>SHMMVSQETVAHVKDLIGQKEVFVAAKTYCPYSKATLSTLFQELNVPKSKALVLELDEMSNGSEIQDALEEISGQKTVPNV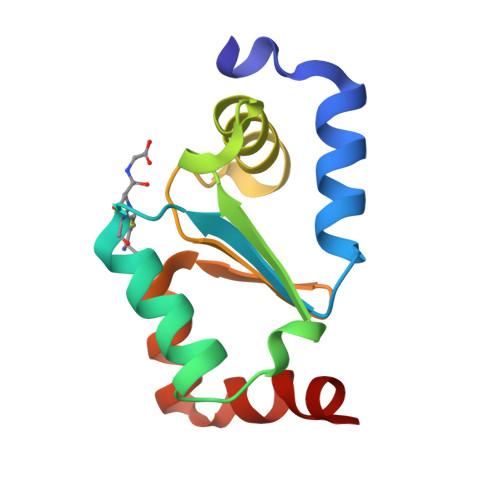YINGKHIGGNSDLETLKKNGKLAEILKPVFQ[2x]> MGSSHHHHHHRVVLRLPERKEVEVKGNRPLREVLEELGLNPETVVAVRGEELLTL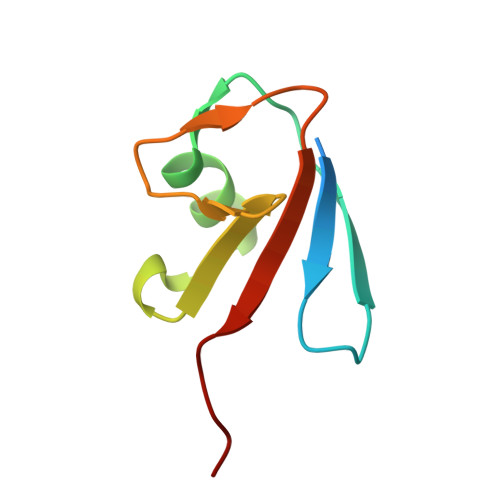EDEVREEDTLEVLSAISGG> AKCVSYGVAQIKAPALHSQGYTGSNVKVAVLDSGIDSSHPDLNVAGGASFVPSETNPFQDNNSHGTHVAGTVLAVAPSASLYAVKVLGADGSGQYSWIINGIEWAIANNMDVINMSL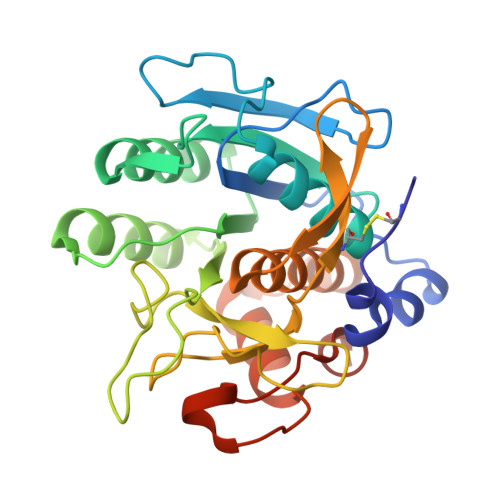GGPSGSAALKAAVDKAVASGVVVVAAAGNNGTSGSSSTVDYPAKYPSVIAVGAVDSSNQRAPWSSVGPELDVMAPGVSICSTLPGGKYGARSGTCGASNHVAGAAALILSKHPNWTNTQVRSSLENTATKLGDSFYYGKGLINVEAAAQHHHHHH> SNAMYIKVCGLTDPHAIDAAQAAHVDAIGFVHAPTSPRHLTPPHI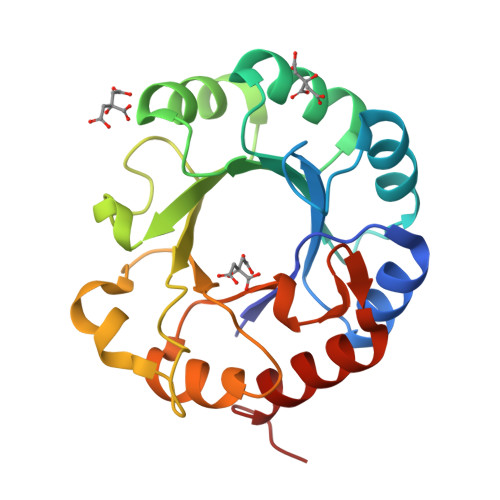STLTATVDCTIDTVLVVATTPIADALALAESTGVSVLQLHGQYSDDDVAYAAARFPRVWRATSLSASPNLTVGAYGEELLLLDAPQAGSGHTWDFAALAHRRPTGRWLLAGGLTPDNVADAITTTSPWGVDVSSGVESAPGVKDPAKIAAFVQAARGVSCPR MESOBILIVERDIN IV ALPHA | C33 H38 N4 O6 | 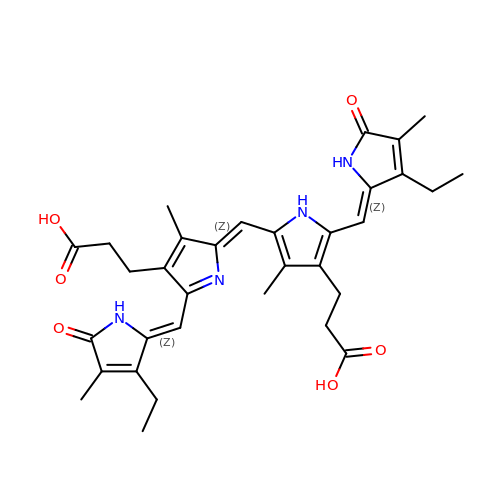OJKQMHYPQBCGFM-BMHFDQIVSA-N The AAA protein Msp1 (in yeast; ATAD1 in mammals) extracts the tail-anchored (TA) membrane proteins that have failed to be correctly inserted into the ER membrane. TA proteins that escape this reaction are mistargeted to the mitochondrial outer membrane (MOM), necessitating their removal. This proofreading function is performed by Msp1/ATAD1, which extracts the mistargeted TA proteins from the MOM to facilitate their subsequent proteasomal degradation. Here, we present a collection of three high-resolution Msp1 solution-state structures (an ATP hydrolysis-arrested Msp1 mutant and two conformational states of wildtype Msp1) that address these outstanding questions and begin to explain how particular features, shared by AAAMC proteins adapt it to its particular roles in protein quality control and beyond. To obtain a homogeneous sample suitable for structural studies, we expressed the cytosolic domain of Msp1 lacking its 30 amino acid N-terminal membrane anchor (Δ30-Msp1) from the thermophilic yeast Chaetomium thermophilum.

We incubated Δ30-Msp1 with ADP•BeFx, an ATP transition state analog that in ATPases (depending on whether BeFx is bound) can mimic both the ATP and the ADP states, and Δ30-Msp1E214Q with ATP. 3D classification of Δ30-Msp1 particles generated two distinct structures: In the first structure the Δ30-Msp1 hexamer adopted the right-handed open spiral arrangement characteristic of AAA proteins (20950 particles analyzed). In the second structure, the Δ30-Msp1 hexamer adopted the same spiral arrangement with the exception of M1, which showed less ordered density, indictive of a continuum of multiple unresolved states in the Msp1 reaction cycle. We fitted M1 into its equilibrium position, in which it closes the seam of the spiral. This structure, henceforth referred to as the ‘closed’ conformation, was based on 48861 particles and resolved to 3.1 Å, approaching 2.5 Å in the stable core. In the open conformation, M1 -M4 were bound to ADP•BeFx (mimicking the ATP state), M5 was bound to ADP, and M6 contained an empty nucleotide-binding pocket. In the closed conformation, each subunit displayed the same nucleotide states, except for M1, for which we could not assign a nucleotide state due to its multiple conformations that resulted in a mostly disordered map. Upon modeling the protein into the density, we observed in all three structures extra density in the central pore of the spiral, spanning its entire depth. This density likely represents an averaged composite of a mixture of peptides from endogenous E. coli proteins that engaged with and became trapped in the central translocation pore. We modeled the putative peptide as poly-alanine with the C-terminus juxtaposed to M1 and its N-terminus to M6.

>GSIAPYLVKIIDPDYEKNERTRIKAQENLRRIRRKQIAEKGDNEDGTDDPSRRRKIDDLVLNEYENQVALEVVAPEDIPVGFNDIGGLDDIIEELKETIIYPLTMPHLYKHGGALLAAPSGVLLYGPPGCGKTMLAKAVAHESGASFINLHISTLTEKWYGDSNKIVRAVFSLAKKLQPSIIFIDEIDAVLGTRRSGEHEASGMVKAEFMTLWDGLTSTNASGVPNRIVVLGATNRINDIDEAILRRMPKQFPVPLPGLEQRRRILELVLRGTKRDPDFDLDYIARVTAGMSGSDIKETCRDAAMAPMREYIRQHRASGKPLSEINPDDVRGIRTEDFFGRRGGKILSEIPPRQTGYVVQSKNSSEGGYEEVEDDDEQGTAST[5x]4-FLUOROPHENOL | 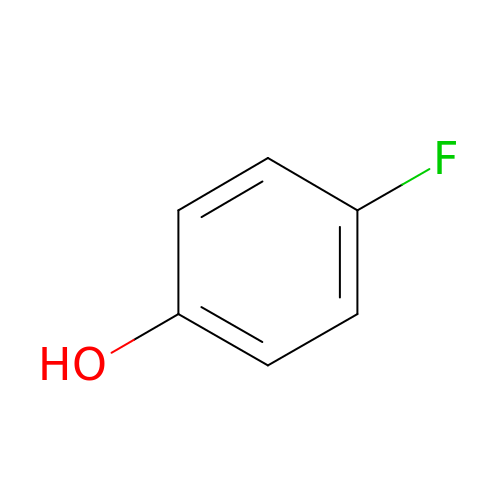C6 H5 F O | RHMPLDJJXGPMEX-UHFFFAOYSA-N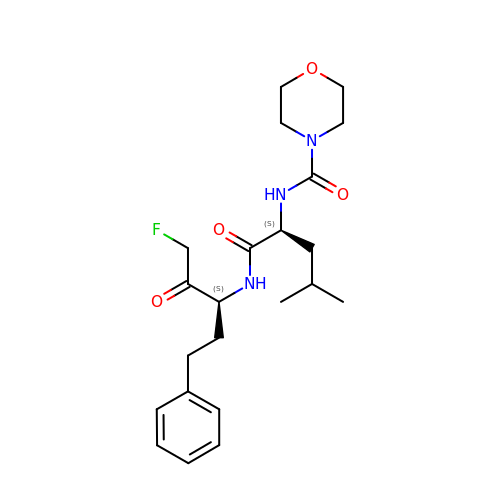N-[(3S)-1-fluoro-2-oxo-5-phenylpentan-3-yl]-N~2~-(morpholin-4-ylcarbonyl)-L-leucinamide | C22 H32 F N3 O4 | DKMMRKMNRYVVBC-OALUTQOASA-N Flavodoxins (Flds) are small flavoproteins of 140–180 amino acids that function as electron carriers in a plethora of redox pathways. They carry a non-covalently bound FMN (flavin mononucleotide) molecule as a prosthetic group, which is able to alternate between three redox states: a completely oxidized state (quinone, Q), a one-electron reduced state (semiquinone, SQ·) and a two-electron reduced state (hydroquinone, HQ). Rhodobacter capsulatus is a non-sulphur purple bacterium capable of fixating atmospheric nitrogen when ammonium levels in the medium are limiting. This microorganism possesses a nitrogen-fixation (nif)-dependent flavodoxin (Rc-NifF) of 181 amino acids, which is included within the long chain subfamily of Flds. In R. capsulatus, nitrogenase reduction by NifF has been proposed to be supported by ferredoxin(flavodoxin)-NADP(H) reductase (FPR, EC 1.18.1.2).

Overall, folding of Rc-NifF is conserved with respect to other flavodoxins, consisting of a central parallel five-stranded beta sheet (β1–β5B) flanked by five alpha helices (α1–α5). Rc-NifF displays the highest structural homology with the long-chain flavodoxin from A. vinelandii with an Rmsd value of 0.55 Å Both present an insertion of eight amino acids at the C-terminal of the 50’s loop (NifF insertion) following the β3 strand (residues 65–72), previously observed in other nif flavodoxins. FMN occupies a cavity located at the C-terminal region of the central β-sheet with the isoalloxazine ring stacked between two hydrophobic residues, the Leu58 (β3–α3 loop) and the Tyr103 (β4–α4 loop). However, while long-chain flavodoxins present a Trp at the re face of the isoalloxazine, nif Flds carries a Leu residue (Leu58 in R. capsulatus). The presence of this Leu at the re face makes the isoalloxazine more accessible to the solvent compared to non-nif Flds containing a Trp in this position, which should provide a major stabilization of the HQ. Rc-NifF was crystallized in the oxydized state, but, unexpectedly, the 50’ loop was found adopting a trans O-up conformation, which should favor FMN reduction in Rc-NifF. Rc-NifF presents a basic patch adjacent to the FMN-binding site formed by Arg16, Lys17 and Lys20 (α1 helix), Lys33 (α1–β2 loop) and Arg39 (β2–α2 loop). These residues introduce large differences in the charge distribution on the surface of the protein, which change the orientation of the dipole moment with respect to other Fld structures reported so far. The eight-residue insertion present in Rc-NifF comprises five backbone carbonyl groups (Leu66, Leu67, Ans69, Ala70 and Ala71) and one side-chain carbonyl group (Asn69) protruding to the solvent.

> MAKIGLFFGSDTGTTRKIAKQIKDMFDDEVMAKPLNVNRADVADFMAYDFLILGTPTLGDGQLPGLSANAASESWEEFLPRIADQDFSGKTIALFGLGDQVTYPLEFVNALFFLHEFFSDRGANVVGRWPAKGYGFEDSLAVVEGEFLGLALDQDNQAALTPERLKGWLSLIAADFGLVLPA> MPCSCASGCQKSKNGGSTPSIRDHVADYYGKTLQSSADLKTSACKLAAAVPESHRKILADIADEVLEKFYGCGSTLPADGSLEGATVLDLGCGTGRDVYLASKLVGEHGKVIGVDMLDNQLEVARKYVEYHAEKFFGSPSRSNVRFLKGFIENLATAEPEGVPDSSVDIVISNCVCNLSTNKLALFKEIHRVLRDGGELYFSDVYADRRLSEAAQQDPILYGECLGGALYLEDFRRLVAEAGFRDVRLVSVGPVDVSDPQLRKLVPDVQFYSCTFRCFKVATLEATREDYGQSATYLGGIGEEFKLDRFFTFPREKPVRVDRNTAEIIRHSRLHQWFSVS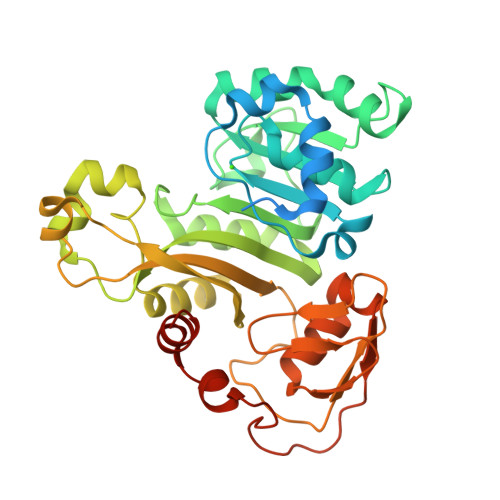AEQQHMGLFKANDSYALLHAPLSMQVEQLVSHHHHHH>[6x]APIKVGINGFGRIGRMVFQAICDQGLIGTEIDVVAVVDMSTNAEYFAYQMKHDTVHGRPKYTVEAVKSSPSVETADVLVVNGHRIKCVKAQRNPADLPWGKLGVDYVIESTGLFTDKLKAEGHIKGGAKKVVISAPASGGAKTIVMGVNQHEYSPASHHVVSNASCTTNCLAPIVHVLTKENFGIETGLMT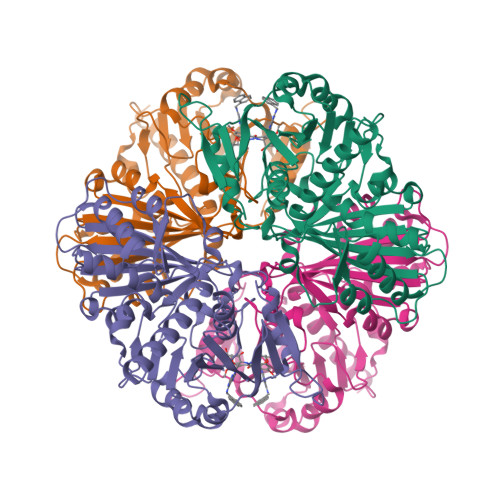TIHSYTATQKTVDGVSLKDWRGGRAAAVNIIPSTTGAAKAVGMVIPSTKGKLTGMSFRVPTPDVSVVDLTFRATRDTSIQEIDKAIKKAAQTYMKGILGFTDEELVSADFINDNRSSVYDSKATLQNNLPGEKRFFKVVSWYDNEWAYSHRVVDLVRYMAAKDAASSKM>GHMSELSVATGAVSTASSSIPMPAGVNPADLAAELAAVVTESVDEDYLLYECDGQWVLAAGVQAMVELDSDELRVIRDGVTRRQQWSGRPGAALGEAVDRLLLETDQAFGWVAFEFGVHRYGLQQRLAPHTPLARVFSPRTRIMVSEKEIRLFDAGIRHREAIDRLLATGVREVPQSRSVDVSDDPSGFRRRVAVAVDEIAAGRYHKVILSRCVEVPFAIDFPLTYRLGRRHNTPVRSFLLQLGGIRALGYSPELVTAVRADGVVITEPLAGTRALGRGPAIDRLARDDLESNSKEIVEHAISVRSSLEEITDIAEPGSAAVIDFMTVRERGSVQHLGSTIRARLDPSSDRMAALEALF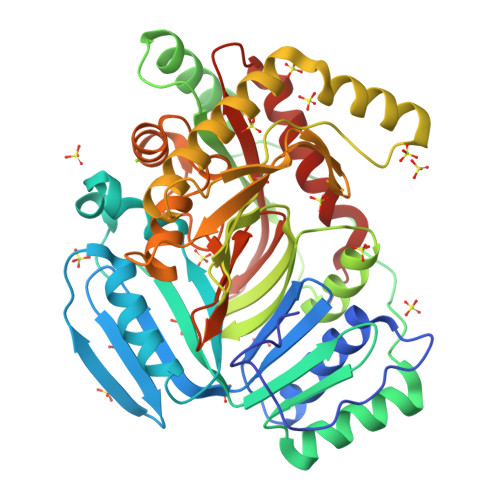PAVTASGIPKAAGVEAIFRLDECPRGLYSGAVVMLSADGGLDAALTLRAAYQVGGRTWLRAGAGIIEESEPEREFEETCEKLSTLTPYLVARQ[4x]> APITAYSQQTRGLLGCIITSLTGRDKNQVEGEVQVVSTATQSFLATCVNGVCWTVYHGAGSKTLAGPKGPITQMYTNVDQDLVGWQAPPGARSLTPCTCGSSDLYL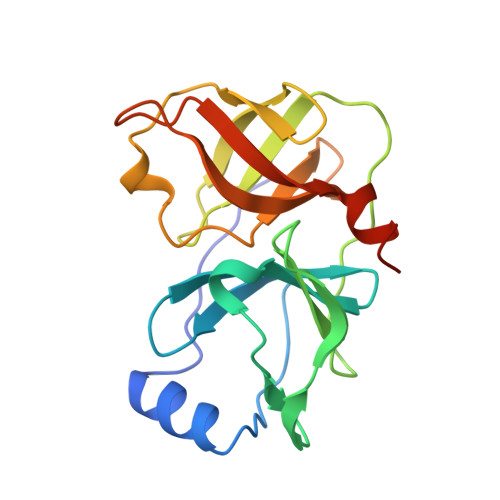VTRHADVIPVRRRGDSRGSLLSPRPVSYLKGSSGGPLLCPSGHAVGIFRAAVCTRGVAKAVDFVPVESMETTMRASKKKK> GSSKQDLMRAVLVEAMTSALNYWERVSGQSKFTFAEQSGLWRVYLDRSTLQTRTLDKYLRIETLPKTPRWRT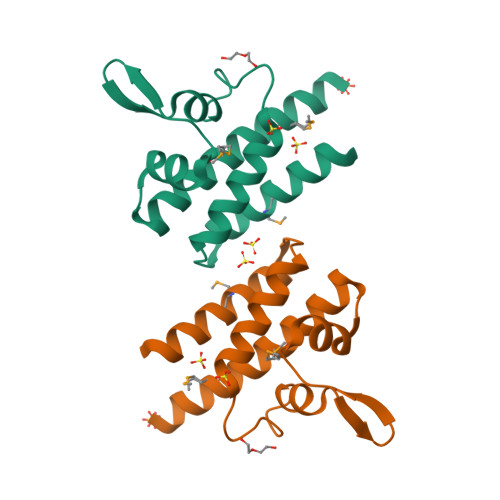VLNSLDYILEHCKEAGPERTHIEMQRDKLQKLLTSE>GSSEPHPVLEKLRSINNYNPKDFDWNLKHGRVFIIKSYSEDDIHRSIKYNIWCSTEHGNKRLDAAYRSMNGKGPVYLLFSVNGSGHFCGVAEMKSAVDYNTCAGVWSQDKWKGRFDVRWIFVKDVPNSQ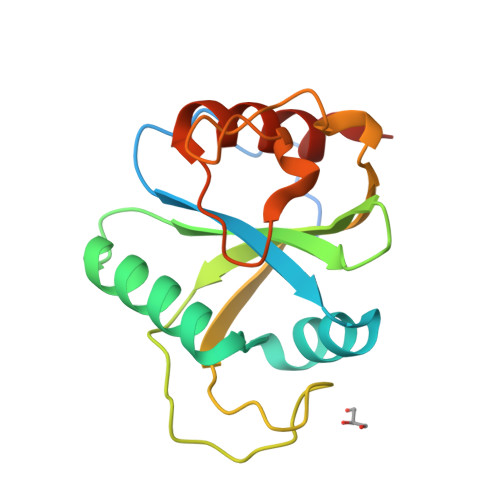LRHIRLENNENKPVTNSRDTQEVPLEKAKQVLKIIASYKHTTSI[2x]> LKESPSGYLRSGEGDTGCGELVWVGEPLTLRTA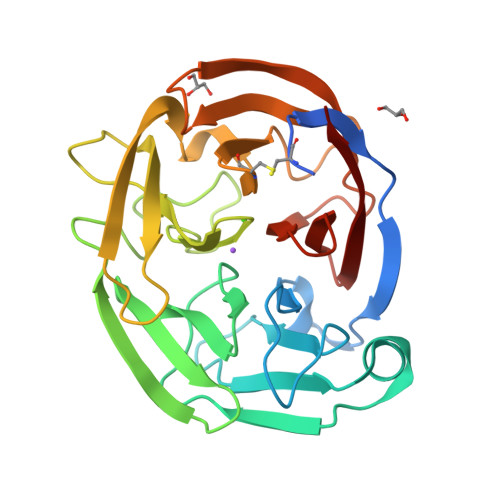ETITGKYGVWMRDPKPTYPYTQETTWRIDTVGKDVRQVFEYDLISQFMQGYPSKVHILPRPLESTGAVVYSGSLYFQGAESRTVIRYELNTETVKAEKEIPGAGYHGQFPYSWGGYTDIDLAVDEAGLWVIYSTDEAKGAIVLSKLNPENLELEQTWETNIRKQSVANAFIICGTLYTVSSYTSADATVNFAYDTGTGISKTLTIPFKNRYKYSSMIDYNPLEKKLFAWDNLNMVTYDIKLSKM> PI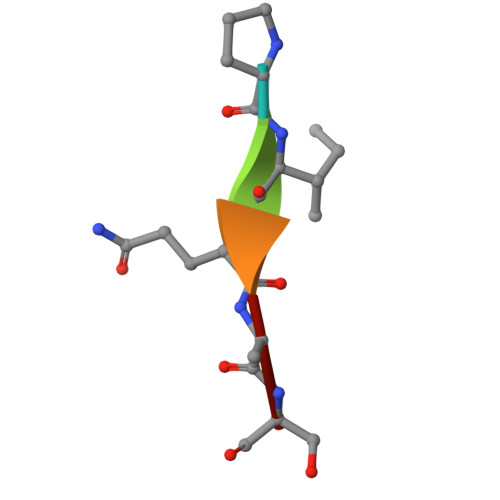QAS> KG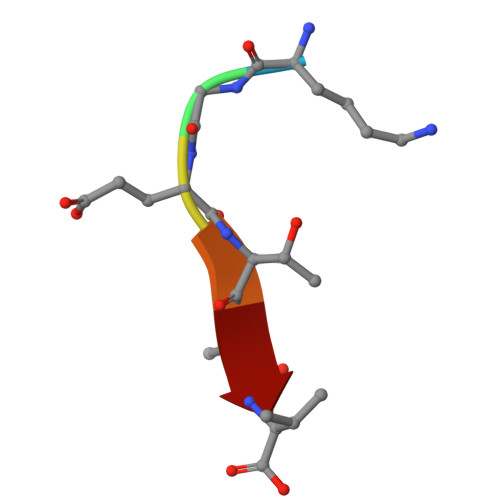ETAV>[8x]MSKRLEGKVALVTGGTSGIGLATAKDLAAQGARVIITGRRQAELDQAVAALGQGVRGVRSDVTRSADLDALFETIRATEGRLDILFTNAGGASMAAL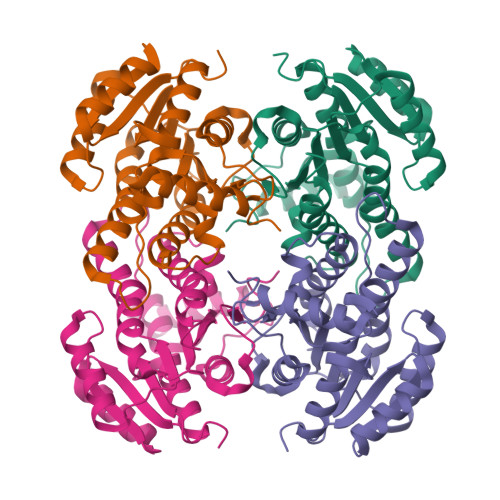GEISEQHFDDTFERNVKAVVFTVQKALPLMPQGASIILNGSIKGSTGTQAFSIYGASKAAVRALARSWVLDLKERGIRVNVVSPGSTRTIGLAELGGDTQEGQDGTLAYLASLVPIGRLADPSEIAKVVSFLASDDSSFINGAEITADGGQAQV>[4x]GSMTSKIALFDQTLIASLLQPLSLNQPDFKAYKTKVKLKI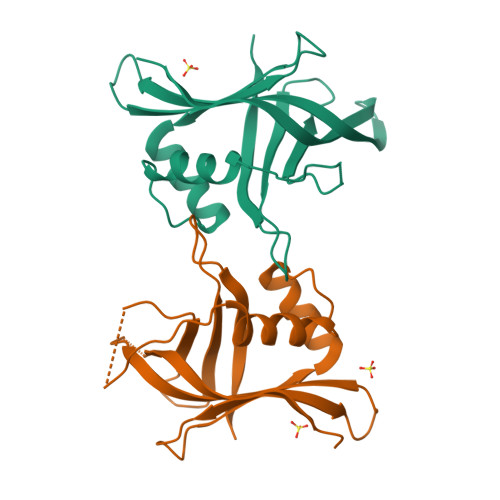SEQRNETSGEKELKFEISRSDDFEFLFSETLNNEKYQILARDHDLTVDFDAFPKVIIQHLLCKNIVKNLEEDGEVDARKKAGYHEIADPGKPTEINIILDAEKNFCSFELFSKTPWSKGKIFSIKLHAVR> VHFKDGVYENIPFKVKGRKTPYALSHFGFFAIGFAVPFVACYV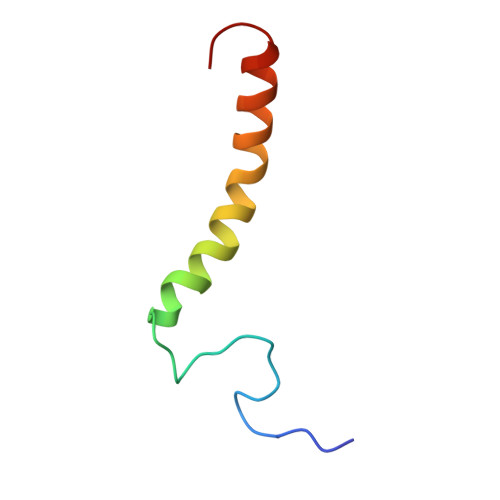QLKKSGAF>[2x]GAMGSTNTTDNIDYFDISDESNYYLISQLRPHFSNIYFFDEFKRYASYHTEIKRYEDIHKTKVNSLLNEASRAIGICNRAKNTVKGLINILENPQKFKTQRESYDVKLRQYEEKKEAFRGCLLNKNRKNLDQIKKINNEIRDLLEKLKCSQDCQTNVYFDMIKIYLVDFKKMPYENYDTFIKQYKN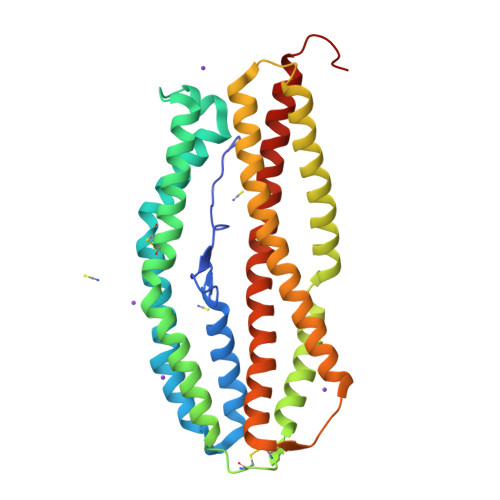SYLSGVDMIRKIEKQIDNPVTINAIKFTQKEMGYIIDRFEYHLQKVKHSIDQVTALSDGVKPKQVTKNRLKEYYFNIGNYYSIFKFGKDSLNMLNKALIHKEKIVHNLLGELFGHLEERIS>MLSRKGIIPEEYVLTRLAEDPAKPRYRARQRRARFVSKKGNCNVAHKNIREQGRFLQDVFTTLVDLKWPHTLLIFTMSFLC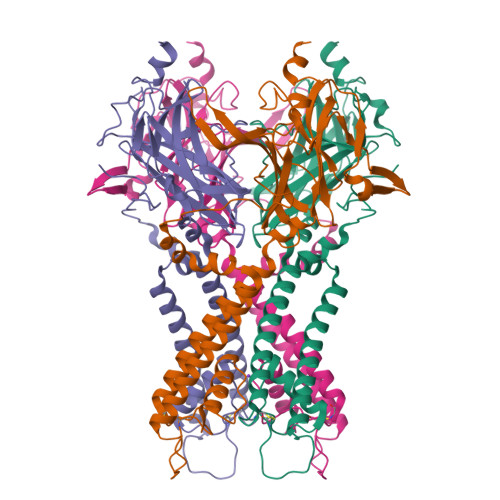SWLLFAMAWWLIAFAHGDLAPSEGTAEPCVTSIHSFSSAFLFSIEVQVTIGFGGRMVTEECPLAILILIVQNIVGLMINAIMLGSIFMKTAQAHRRAETLIFSKHAVIALRHGRLCFMLRVGDLRKSMIISATIHMQVVRKTTSPEGEVVPLHQVDIPMENGVGGNSIFLVAPLIIYHVIDANSPLYDLAPSDLHHHQDLEIIVILEGVVETTGITTQARTSYLADEILWGQRFVPIVAEEDGRYSVDYSKFDNTVKVPTPLCTARQLDEDHSLLEALTLASARGPLRKRSVPMAKAKPKFSISPDSLS[4x]> TGV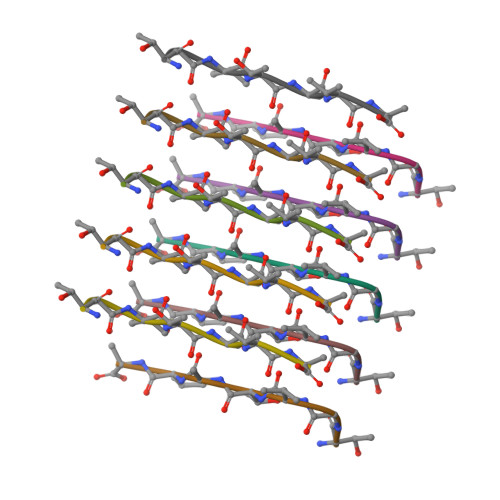TAVA> WATSEPSYPSPWMNPNAAGWEQAYQWAKDFVSQMTLLEKVNLTTGVGWEGEQCVGQTGAIPRLGLRSLCLHDSPLGIRGTDYNSAFPSGQTTAATWDRTLFYKRGYAMGKEARGKGINVLLGPVAGPLGRMPAGGRNWEGFSPDPVLTGIAMAETVKGIQDAGVIACAKHLIGDEQEHFRQVGDGFDIDESLSSNIDDRTMHELYLWPFADAVRAGVGSVMCAYNQVNNSYSCHNSKLLNGLLKNELGFQGFVMSDWQAQ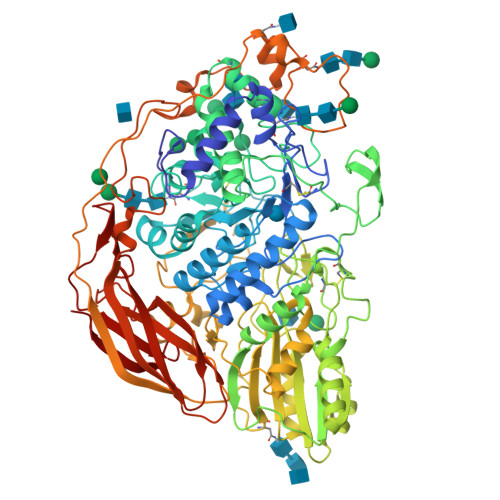HTGVASAVAGLDMTMPGDTVFNSGLSFWGANLTVAVLNGTLPAYRLDDMAMRIMAAFFKVRGTQDVDLDPINFSFWTLDTYGPIHWGAKEGHQQINFHVDVREDHSRLIREIAAKGTVLLKNEGALPLDKPKFLAVIGEDAGPNHNGPNSCDDRGCVGGTLAMGWGSGTANFPYLVTPDAALQAQAIKDGSRYESVLSNHAMETIRKVVSQDNVTAVVFVNANSGEGYITVDGNRGDRNNLTLWNGGDELIKNVASWCSNTIVVIHSVGPVLLTDWYDHPNITAILWAGLPGQESGNAITDVLYGKVNPAGRSPFTWGATREGYGADVLYDPDDARVPQQNFTEGVFIDYRYFDKHNTRVIYEFGHGLSYTTFEYRNLQIQKHNVSAYIPTTGLTEPAPTFGEHSTNYSDYLYPEGFHRANRYIYPYVNSTDLELASGDPYYGQTADQFLPPNATSSDPQPLLRSSGKNSPGGNPQLYDVLYTVTADITNTGALEGDEVVQLYVSLGGPDDPKVMLRDFARLHIKPGETVKFEGKLTRRDLSTWDVTLQDWVIRDHTKMVFLGKSSRKLVLGALLN>MVLYFIGLGLYDERDITVKGLEIAKKCDYVFAEFYTSLMAGT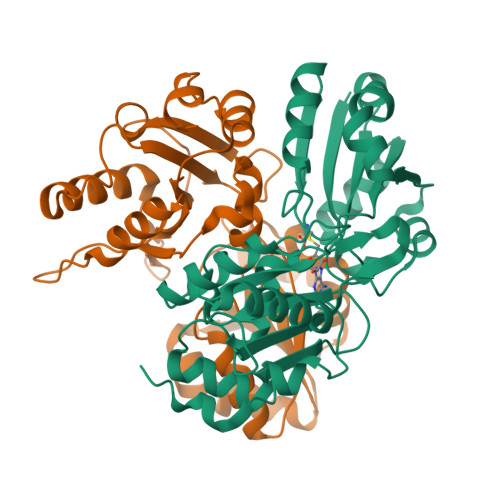TLGRIQKLIGKEIRVLSREDVELNFENIVLPLAKENDVAFLTPGDPLVATTHAELRIRAKRAGVESYVIHAPSIYSAVGITGLHIYKFGKSATVAYPEGNWFPTSYYDVIKENAERGLHTLLFLDIKAEKRMYMTANEAMELLLKVEDMKKGGVFTDDTMVVVLARAGSLNPTIRAGYVKDLIREDFGDPPHILIVPGKLHIVEAEYLVEIAGAPREILRVNV[2x]>MVAAPPAVGAAMPSLDFDTSVFNKEKVSLAGHEEYIVRGGRNLFPLLPEAFKGIKQIGVIGWGSQGPAQAQNLRDSLAEAKSDIVVKIGLRKGSKSFDEARAAGFTEESGTLGDIWETVSGSDLVLLLISDAAQADNYEKIFSHMKPNSILGLSHGFLLGHLQSAGLDFPKNISVIAVCPKGMGPSVRRLYVQGKEINGAGINSSFAVHQDVDGRATDVALGWSVALGSPFTFATTLEQEYKSDIFGERGILLGAVHGIVEALFRRYTEQGMDEEMAYKNTVEGITGIISKTISKKGMLEVYNSLTEEGKKEFNKAYSASFYPCMDILYECYEDVASGSEIRSVVLAGRRFYEKEGLPAFPMGNIDQTRMWKVGEKVRSTRPENDLGPLHPFTAGVYVALMMAQIEVLRKKGHSYSEIINESVIESVDSLNPFMHARGVAFMVDNCSTTARLGSRKWAPRFDYILTQQAFVTVDKDAPINQDLISNFMSDPVHGAIEVCAELRPTVDISVPANADFVRPELRQSS[2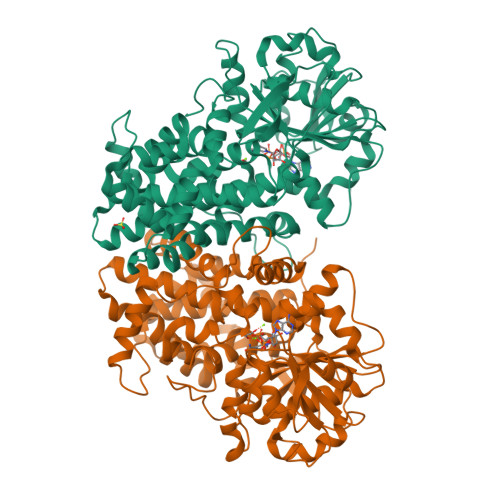x]>[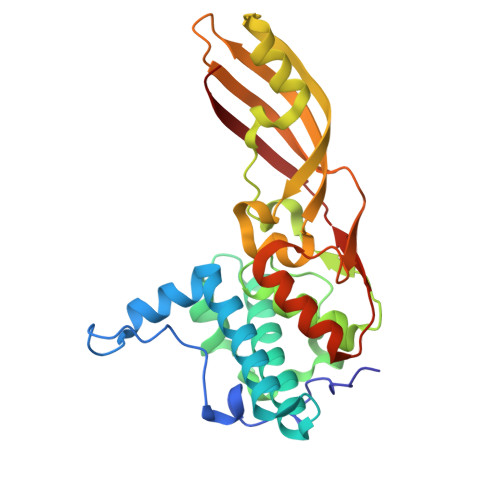2x]METLTVHAPSPSTNLPSYGNGAFSLSAPHVPGAGPLLVQVVYSFFQSPNMCLQALTQLEDYIKKHGASNPLTLQIISTNIGYFCNADRNLVLHPGISVYDAYHFAKPAPSQYDYRSMNMKQMSGNVTTPIVALAHYLWGNGAERSVNIANIGLKISPMKINQIKDIIKSGVVGTFAVSTKFTHATGDYNVITGAYLGNITLKTEGTLTISANGSWTYNGVVRSYDDKYDFNASTHRGIIGESLTRLGAMFSGKEYQILLPGEIHIKESGKR>ATAVNGAPRDAALWSSHEQMLAQPLKDSDAEVYDIIKKESNRQRVGLELIASENFASRAVLEALGSCLNNKYSQGYPGQRYYGGTEHIDELETLCQKRALQAYGLDPQCWGVNVQPYSGSPANFAVYTALVEPHGRIMGLDLPDGGHLTHGFMTDKKKISATSIFFESMAYKVNPDTGYIDYDRLEENARLFHPKLIIAGTSCYSRNLDYGRLRKIADENGAYLMADMAHISGLVVAGVVPSPFEHCHVVTTTTHKTLRGCRAGMIFYRRGVRSVDPKTGKEILYNLESLINSAVFPGLQGGPHNHAIAGVAVALKQAMTPEFKEYQRQVVANCRALSAALVELGYKIVTGGSDNHLILVDLRSKGTDGGRAEKVLEACSIAC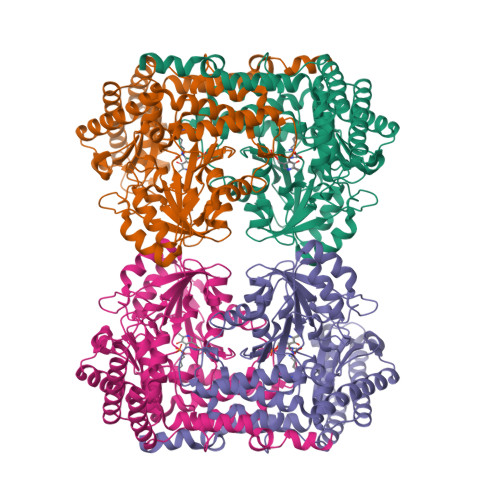NKNTCPGDKSALRPSGLRLGTPALTSRGLLEKDFQKVAHFIHRGIELTVQIQDDTGPRATLKEFKEKLAGDEKHQRAVRALRQEVESFAALFPLPGLPGF[2x]>MTEYNSEAYLKKLDKWWRAATYLGAGMIFLKENPLFSVTGTPIKAENLKANPIGHWGTVSGQTFLYAHANRLINKYDQKMFYMGGPGHGGQAMVVPSYLDGSYTEAYPEITQDLEGMSRLFKRFSFPGGIGSHMTAQTPGSLHEGGELGYVLSHATGAILDQPEQIAFAVVGDGEAETGPLMTSWHSIKFINPKNDGAILPILDLNGFKISNPTLFARTSDVDIRKFFEGLGYSPRYIENDDIHDYMAYHKLAAEVFDKAIEDIHQIQKDAREDNRYQNGEIPAWPIVIARLPKGWGGPRYNDWSGPKFDGKGMPIEHSFRAHQVPLPLSSKNMGTLPEFVKWMTSYQPETLFNADGSLKEELRDFAPKGEMRMASNPVTNGGVDSSNLVLPDWQEFANPISENNRGKLLPDTNDNMDMNVLSKYFAEIVKLNPTRFRLFGPDETMSNRFWEMFKVTNRQWMQVIKNPNDEFISPEGRIIDSQLSEHQAEGWLEGYTLTGRTGAFASYESFLRVVDSMLTQHFKWIRQAADQKWRHDYPSLNVISTSTV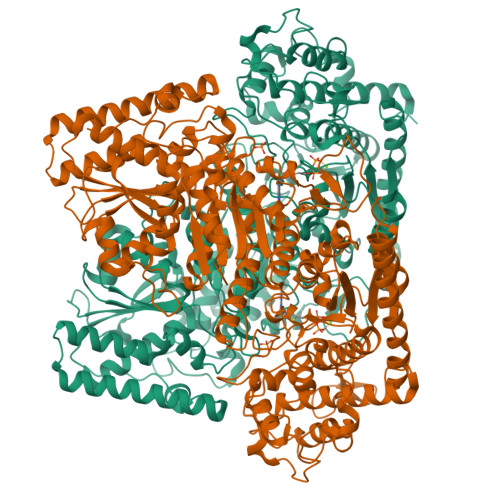FQQDHNGYTHQDPGMLTHLAEKKSDFIRQYLPADGNTLLAVFDRAFQDRSKINHIVASKQPRQQWFTKEEAEKLATDGIATIDWASTAKDGEAVDLVFASAGAEPTIETLAALHLVNEVFPQAKFRYVNVVELGRLQKKKGALNQERELSDEEFEKYFGPSGTPVIFGFHGYEDLIESIFYQRGHDGLIVHGYREDGDITTTYDMRVYSELDRFHQAIDAMQVLYVNRKVNQGLAKAFIDRMKRTLVKHFEVTRNEGVDIPDFTEWVWSDLKK[8x]>LTLGNTTSSVILTNYMDTQYYGEIGIGTPPQTFKVVFDTGSSNVWVPSSKCSRLYTACVYHKLFDASDSSSYKHNGTELTLRYSTGTVSGFLSQDIITVGGITVTQMFGEVTEMPALPFMLAEFDGVVGMGFIEQAIGRVTPIFDNIISQGVLKEDVFSFYYNRDS[2x];>SLGGQIVLGGSDPQHYEGNFHYINLIKTGVWQIQMKGVSVGSSTLLCEDGCLALVDTGASYISGSTSSIEKLMEALGAKKRLFDYVVKCNEGPTLPDISFHLGGKEYTLTSADYVFQESYSSKKLCTLAIHAMDIPPPTGPTWALGATFI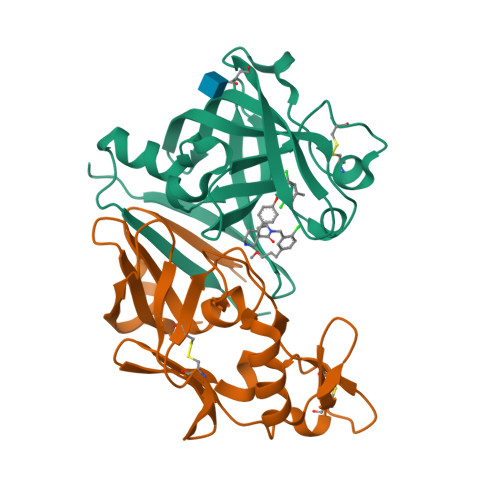RKFYTEFDRRNNRIGFALARHHHHHH[2x]>[2x]MLPQRLHPSRLLALALF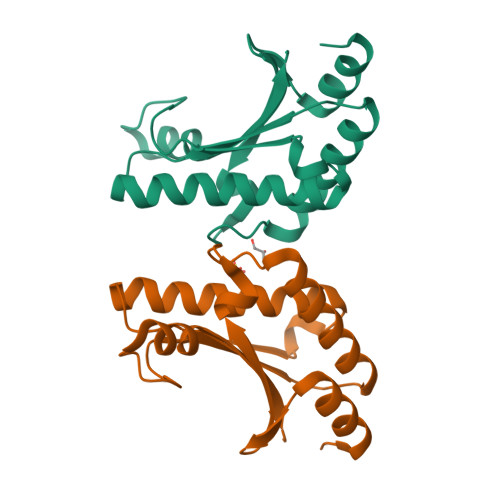SLVLGLAGCQTKPPQTGLSAEQIAVLQEQGFELRDEGLEFGMSSKVLFGNNLDRLNPDSRNTLTKIARALLAVDIDKVRLEGHTDNYGDEGYNQKLSERRAESVAAVFREAGMPAANIEVRGLGMSKPVADNKTRAGRSENRRVAIIVPAE>GSHMTAPVVRNPEVYNRTQFPIFHWCRGGKALSMLPKFDTYGQSKVEINIVGSGGGSGGGSVTIGNAHDDLIHDAVLDYYGRRLATCSSDKTIKIFEIDGENQRLVETLIGHEGPVWQVAWAHPKFGVILASCSYDGKVLIWKEDNGVWNKVAEHSVHQASVNSVSWAPHEYGPVLLCASSDGKISIVEFKDGGALEPIVIQGHAIGVNAASWAPISLPDNTRRFVSGGCDNLVKIWRYDDAAKTFIEEEAFQGHSDWVRDVAWSPSRLSKSYIATASQDRTVLIWTKDGKSNKWEKQPLTKEKFPDVCWRASWSLSGNVLAISGGDNKVTLWKENIQGKWE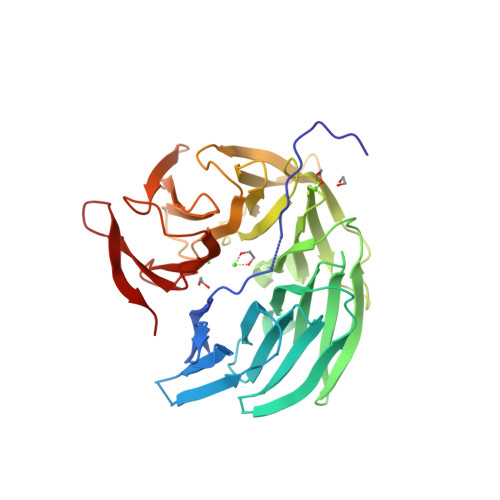SAGEVDQ[2x]>[3x]MEHSSLETI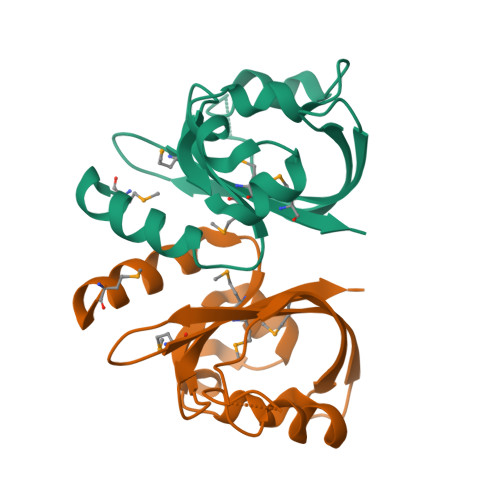ELFIQHLTEAMILVNANGFIRSCNQRSAELLDCPQVSLKGQDWRNFLTEHHQARYDNLLSHDVQLGTNCGQPVQHPAQETTLICASGKAKDVELSISYIPGHEPMFVMVMHDLEHHHHHH>YFQGMITEFLLKKKLEEHLSHVKEENTIYVTDLVRCPRRVRYESEYKELAISQVYAPSAILGDILHLGLESVLKGNFNAETEVETLREINVGGKVYKIKGRADAIIRNDNGKSIVIEIKTSRSDKGLPLIHHKMQLQIYLWLFSAEKGILVYITPDRIAEYEINEPLDEATIVRLAEDTIMLQNSPRFNWECKYC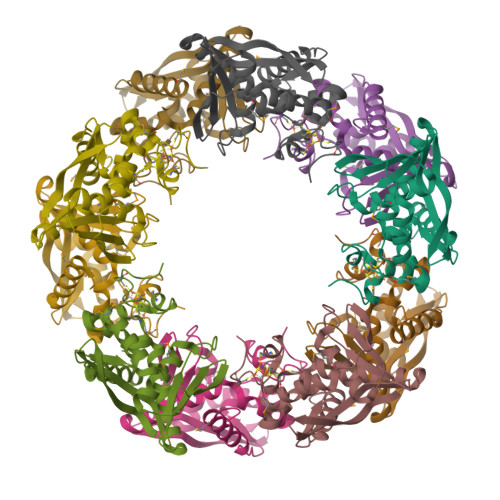IFSVICPAKLT[10x]>[2x]MMSETAPLPSASSALEDKAASAPVVGIIMGSQSDWETMRHADALLTELEIPHETLIVCAHRTPDRLADYARTAAERGLNVIIAGAGGAAHLPGMCA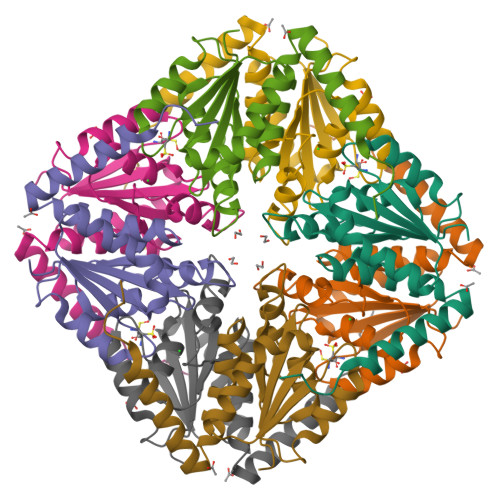AWTRLPVLGVPVESRALKGMDSLLSIVQMPGGVPVGTLAIGASGAKNAALLAASILALYNPALAARLETWRALQTASVPNSPITEDK> MFRSTRPRSVGYTPVNPDTSPMVAYSQYHWHYNLPQGMERPHSVNRTFAAPFQSNHSLVNKYRGVWIEFDMHPAFSVALEPQLRKLPRGRTLPKTPAEEVIADYTALAPLVDDEKTRDLWLAKVFQHCAFQRCGGAMELWERYCHQRFTAEG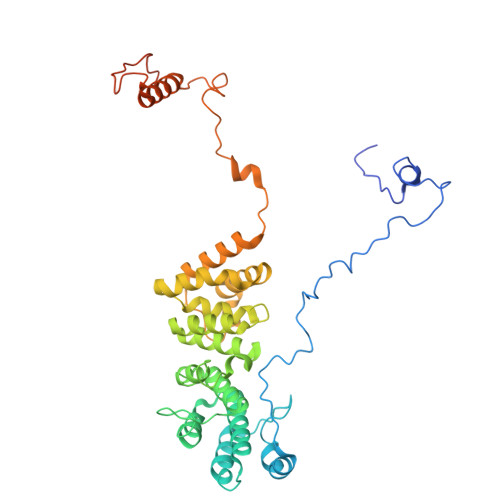ATAKPPLSLVKSVLFYCNKTDNSGWRALFDRCLKDGWNYTPLFDTAQWSFMLKSIGRMGDEDGVRAVLEEMLDVQADLDRVEARSVVIALNAVTNADVYEFVKKYLFNFGERKVKFLRTTYSDLRGHGAGKLRIPLKENDNMYYHVCWHSSIRSPRQFSPRQLYFDYTPSTLGSSSHNPNAKIDDIVKDKIEKWKAEGLLPEDYVHEDRVYDRSAAFKNVARQEKWKKMPKILKSKRMGYTGDP> GSTRYVPYTI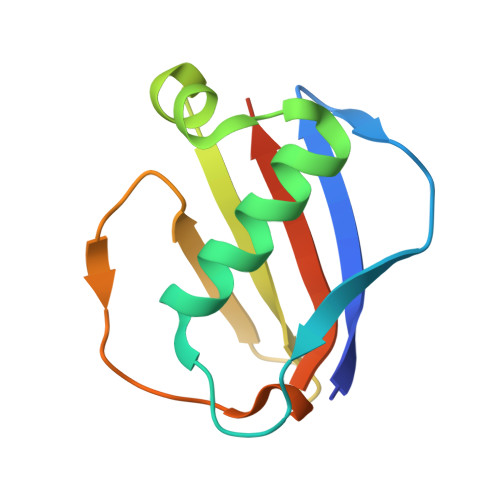AVNGTSTPILSKLKISNKQLISYKYLNDKVKSVLKSERGISDLDLKFAKQAKYTVYFKNGKKQVVNLKSDIFTPNLFSAKDIKKIDIDVKQYTKSKKK>MHHHHHHGSMSMPNHQNMLDNQTILITGGTGSFGKCFVRKVLDTTNAKKIIVYSRDELKQSEMAMEFNDPRMRFFIGDVRDLERLNYALEGVDICIHAAALKHVPIAEYNPLECIKTNIMGASNVINACLKNAISQVIALSTDKAANPINLYGATKLCSDKLFVSANNFKGSSQTQFSVVRYGNVVGSRGSVVPFFKKLVQNKASEIPITDIRMTRFWITLDEGVSFVLKSLKRMHGGEIFVP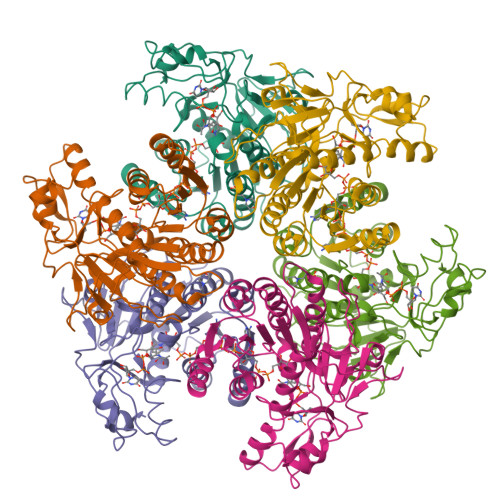KIPSMKMTDLAKALAPNTPTKIIGIRPGEKLHEVMIPKDESHLALEFEDFFIIQPTISFQTPKDYTLTKLHEKGQKVAPDFEYSSHNNNQWLEPDDLLKLL[2x]> MHHHHHHSGRSVANQANLIDNKRELEQHALVPYAQGKSIHQLFEEQAEAFPDRVAIVFENRRLSYQELNRKANQLARALLEKGVQTDSIVGVMMEKSIENVIAILAVLKAGGAYVPIDIEYPRDRIQYILQDSQTKIVLTQKSVSQLVHDVGYSGEVVVLDEEQLDARE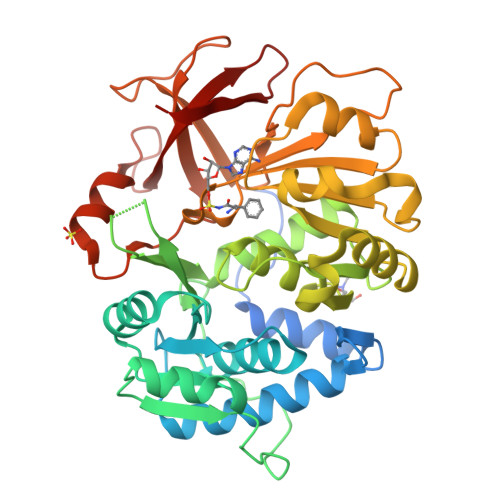TANLHQPSKPTDLAYVIYTSGTTGKPKGTMLEHKGIANLQSFFQNSFGVTEQDRIGLFASMSFDVSVWEMFMALLSGASLYILSKQTIHDFAAFEHYLSENELTIITLPPTYLTHLTPERITSLRIMITAGSASSAPLVNKWKDKLRYINAYGPTECLVATIWEAPSNQLSVQSVPIGKPIQNTHIYIVNEDLQLLPTGSEGELCIGGVGLARGYWNRPDLTAEKFVDNPFVPGEKMYRTGDLAKWLTDGTIEFLGRI>[4x]PDIFNRDPRDHYDLLQRLGGGTYGEVFKARDKVSGDLVALKMVKMEPDDDVSTLQKEILILKTCRHANIVAYHGSYLWLQKLWIC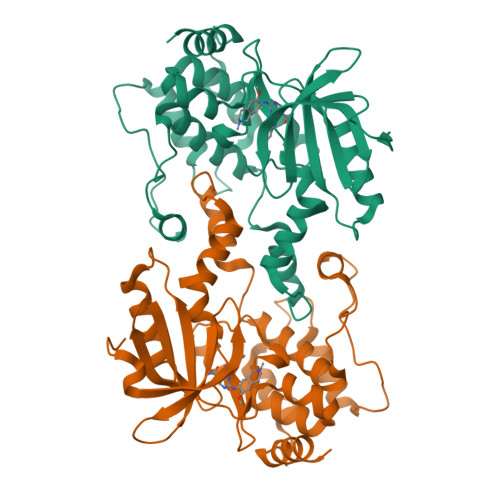MEFCGAGSLQDIYQVTGSLSELQISYVCREVLQGLAYLHSQKKIHRDIKGANILINDAGEVRLADFGISAQIGAELARRLEFIGTPYWMAPEVAAVALKGGYNELCDIWSLGITAIELAELQPPLFDVHPLRVLFLMTKSGYQPPRLKEKGKWSAAFHNFIKVTLTKSPKKRPSATKMLSHQLVSQPGLNRGLILDLLDKLKNP> LPTSNPAQELEARQLGRTTRDDLINGNSASCADVIFIYARGSTETGNLGTLGPSIASNLESAFGKDGVWIQGVGGAYRATLGDNALPRGTSSAAIREMLGLFQQANTKCPDATLIAGGYCQGAALAAASIEDLDSAIRDKIAGTVLFGYTKNLQNRGRIPNYPADRTKVFCNTGDL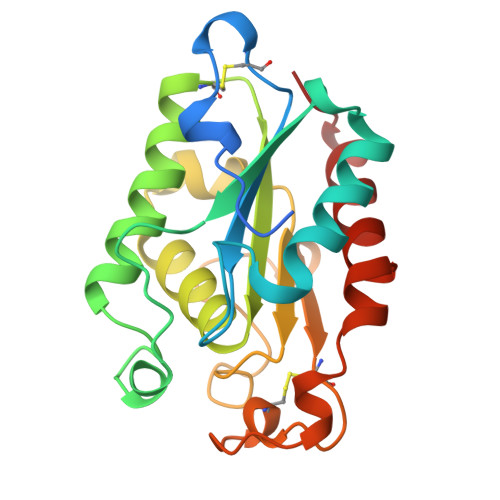VCTGSLIVAAPHLAYGPDARGPAPEFLIEKVRAVRGSA>[2x]MGSSHHHHHHSSGLVPRGSHMEAPAAPAAEAPAAGTESGMAAGLVAWPLSARGERALRGQAGRLADWADAGTGLSATASALVHRRSALEHRAVVTADSL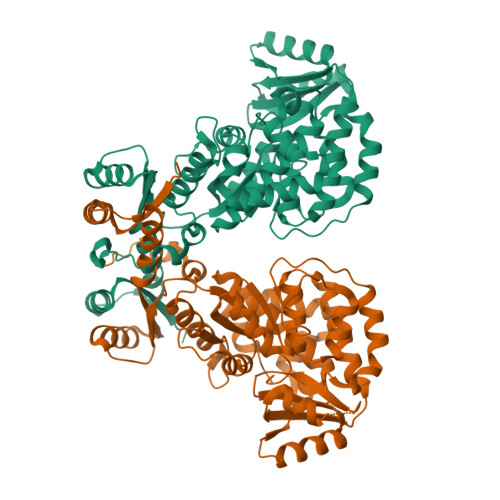EGQLAALRALAAGEEAPGLRQGQLPATQGRLAFLFSGQGAQRAGMGRELYAAEPVFAAAFDEVCAAFGEDLRERIFTARQEELDRTGTTQPALFAIEVALFRLVESLGVRPDFVAGHSIGELAAAHVAGVLSLPDACRLVAARGQLMEALPEGGAMVSVRATEDEVRAHLAEFTGRVDVAAVNGPESVVLSGEEAAVEEIAGRLAEAGRKTRRLRVSHAFHSPLMEPMLDAFRRVAEELTYQAPSVPVVSNLTGEQVTAFDAAYWVEHVRRAVRFADGIGFLASRGVTRFVELGPDGVLTAMAQETLTDPETLLLPVLRKDRPEPEAFLDALAQAWTRGVDVDWAARYGPEQSTGVSLPTYAFQ N-{[(3R,5S)-7-chloro-5-(2,3-dimethoxyphenyl)-1-(2,2-dimethylpropyl)-2-oxo-1,2,3,5-tetrahydro-4,1-benzoxazepin-3-yl]acetyl}-L-aspartic acid | C28 H33 Cl N2 O9 | 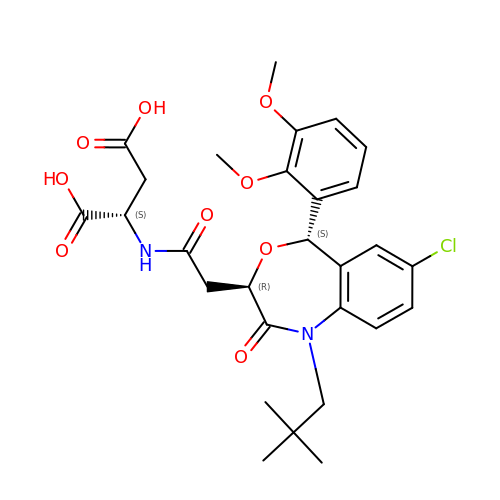RKWDCULOIHHIST-SNYIIPAISA-N The discoidin domain receptors (DDRs), DDR1 and DDR2, are unique among the receptor tyrosine kinases (RTKs) in being activated by interaction with the extracellular matrix. A single transmembrane helix links to the cytoplasmic domain, where a larger JM region precedes the catalytic C-terminal kinase domain. Overall, DDR1 displays the classical bilobal architecture of a tyrosine kinase. As observed for ABL, both type II inhibitors induce an inactive conformation of DDR1 characterized by a “DFG-Asp out, αC-Glu in” configuration.

The DDR1–imatinib complex structure was solved subsequently using data collected from crystals improved by microseeding procedures. The structure was solved by molecular replacement and refined to 1.7 Å resolution. Disordered regions in the imatinib co-structure were identified in both the KID region and a portion of the activation segment spanning residues 799–803. DDR1 was monomeric in the imatinib complex, consistent with its size-exclusion profile, whereas the ponatinib complex formed a crystallographic dimer with an additional ponatinib molecule bound at the dimer interface. In total, imatinib forms six hydrogen bonds in the ATP pocket of DDR1. Two target the hinge region, including one between the pyridine head group and the backbone amide of Met704 and one between the aminopyrimidine and the gatekeeper residue Thr701. Two more are made by the linker: the amide binds to Glu672 in the αC, while the carbonyl contacts the backbone amide of Asp784 in the DFG motif. Finally, the methylpiperazine group occupies a hydrophobic pocket between the αC and HRD (His-Arg-Asp) motif and hydrogen bonds with the backbone carbonyls of Val763 and His764. The DFG motif further stabilizes the binding with a π–π stacking interaction between Phe785 and the aminopyrimidine group. The strong binding of DDR1 to imatinib was revealed by isothermal titration calorimetry (ITC), which indicated a dissociation constant (KD) of 1.9 nM.

>[2x]SMPRVDFPRSRLRFKEKLGEGQFGEVHLCEVDSPQDLVSLDFPLNVRKGHPLLVAVKILRPDATKNARNDFLKEVKIMSRLKDPNIIRLLGVCVQDDPLCMITDYMENGDLNQFLSAHQLEDKAAEGAPGDGQAAQGPTISYPMLLHVAAQIASGMRYLATLNFVHRDLATRNCLVGENFTIKIADFGMSRNLYAGDYYRVQGRAVLPIRWMAWECILMGKFTTASDVWAFGVTLWEVLMLCRAQPFGQLTDEQVIENAGEFFRDQGRQVYLSRPPACPQGLYELMLRCWSRESEQRPPFSQLHRFLAEDALNTV>GPLGSRPWQILSQALGFPNYDQELWWQNTAETLNRVLEQCDYSVHLQYKYLAFYHKYILPSLGPFRRPGVEPEYISGLSHGGHPLEISVKIDKSKTICRLGLQAIGPLAGTARDPLNSFGDRELLKNLATLLPHVDLRLFDHFNAQVGLDRAQCAVATTKLIKESHNIVCTSLDLKDGEVIPKVYFSTIPKGLVTETPLFDLTFAAIEQMEVYHKDAPLRTALSSLKDFLRPRVPTDASITPPLTGLIGVDCIDPMLSRLKVYLATFRMDLSLIRDYWTLGGLLTDAGTMKGLEMVETLAKTLKLGDEACETLDAERLPFGINYAMKPGTAELAPPQIYFPLLGINDGFIADALVEFFQYMGWEDQANRYKDELKAKFPNVDISQTKNVHRWLGVAYSE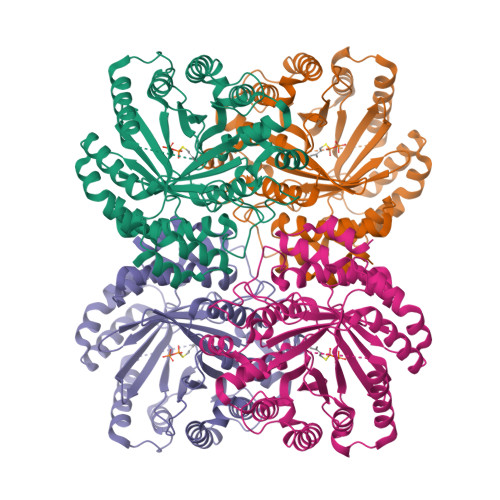TKGPSMNIYYDVVAGNVARV[2x]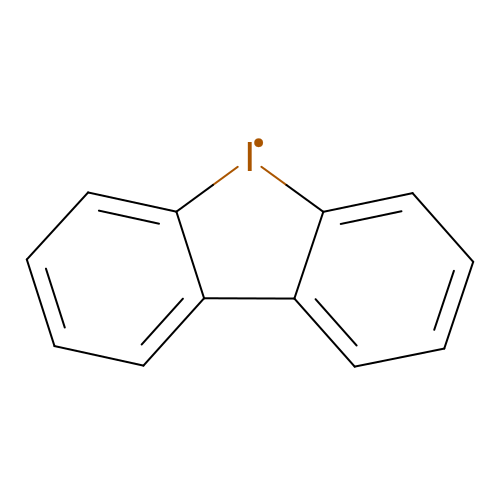benzo[b][1]benziodole | C12 H8 I | PEWVMQDYYUSPRM-UHFFFAOYSA-N>[2x]ATVPLPAEGEIGLVHIGALTLENGTVLPDVTIAVQRWGELAPDRGNVVMVLHALTGDSHVTGPAGDGHPTAGWWDGVAGPGAPIDTDHWCAIATNVLGGCRGSTGPGSLAPDGKPWGSRFPQITIRDQVAADRAALAALGITEVAAVVGGSMGGARALEWLVTHPDDVRAGLVLAVGARATADQIGTQSTQVAAIKADPDWQGGDYHGTGRAPTEGMEIARRFAH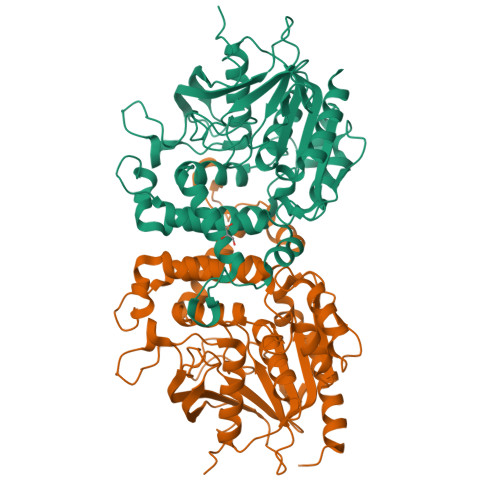LTYRGEEELDDRFANTPQDDEDPLTGGRYAVQSYLEYQGGKLARRFDPGTYVVLSDALSSHDVGRGRGGVEAALRSCPVPVVVGGITSDRLYPIRLQQELAELLPGCQGLDVVDSIYGHDGFLVETELVGKLIRRTLELAQRLEHHHHH> MVLHKWAVVSRSAPPPRGLRPIARTIPTHPRLRPVDYKIPYVLRTFIKDRHTSE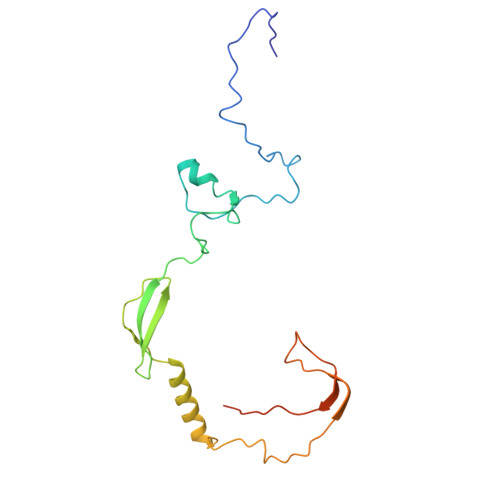VQHLENRGMFAEELSIERSRFPRFHSTFTIQTDGSLNEREFEFAVPPIVTLFHDRLSAHRERQLELAKIGKLRKERNWETEQKGEESVSMACNALAFPYCIPKNMLKRSRVVDPLNSKSSTQGVTSGGG5-[(3S)-5,5-dimethyloxolan-3-yl]-6-methoxy-3-(2-methoxypyridin-4-yl)pyrazolo[1,5-a]pyrimidine | C19 H22 N4 O3 | 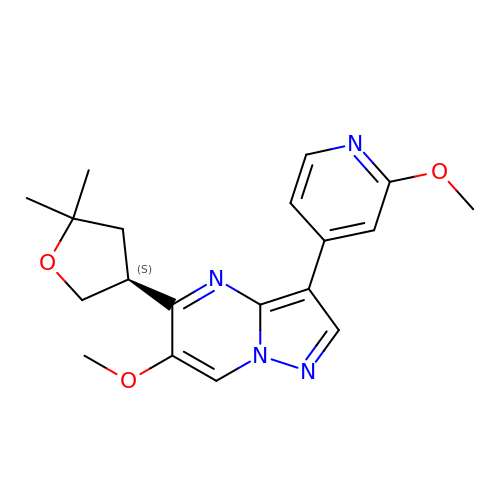PETJVBHONPBYQW-CYBMUJFWSA-N> MLEMATVEPETTPTPNPPTTEEEKTESNQEVANPEHYIKHPLQNRWALWFFKNDKSKTWQANLRLISKFDTVEDFWALYNHIQLSSNLMPGCDYSLFKDGIEPMWEDEKNKRGGRWLITLNKQQRRSDLDRFWLETLLCLIGESFDDYSDDVCGAVVNVRAKGDKIAIWTTECENREAVTHIGRVYKERLGL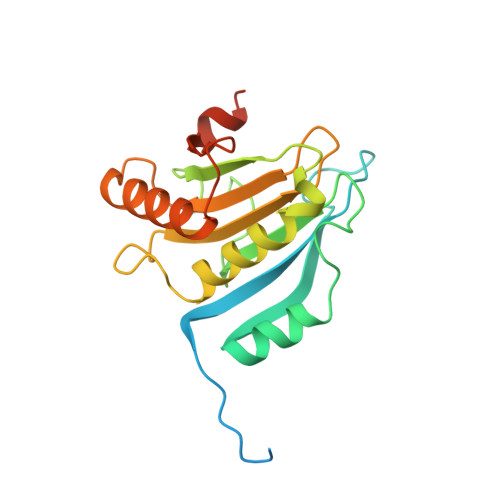PPKIVIGYQSHADTATKSGSTTKNRFVV> MSYGKGNVFAYRTYLKPLTGVKQIPESSFAGRDNTVVGVDVTCEIGGEAFLPSFTDGDNTLVVATDSMKNFIQRHLASYEGTTTEGFLHYVAHRFLDTYSHMDTITLTGEDIPFEAMPAYEEKELSTSRLVFRRSRNERSRSVLKAERSGNTITITEQYSEIMDLQLVKVSGNSFVGFIRDEYTTLPEDGNRPLFVYLNISWQYENTNDSYASDPARYVAAEQVRDLASTVFHELETPSIQNLIYHIGCRILARFPQLTDVSFQSQ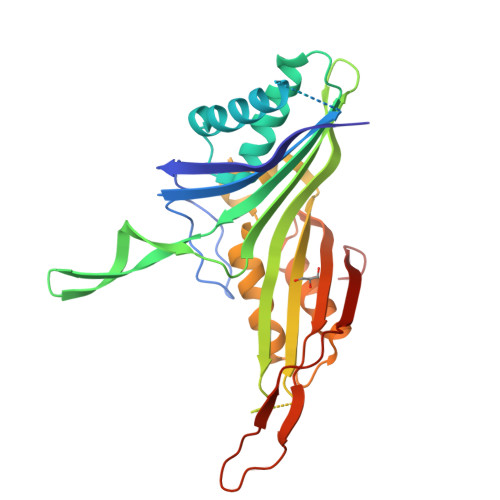NHTWDTVVEEIPGSKGKVYTEPRPPYGFQHFTVTREDAE>GSAAKMAKNVDKPLFTATFNVQASSADYATFIAGIRNKLRNPAHFSHNRPVLPPVEPNVPPSRWFHVVLKASPTSAGLTLAIRADNIYLEGFKSSDGTWWELTPGLIPGATYVGFGG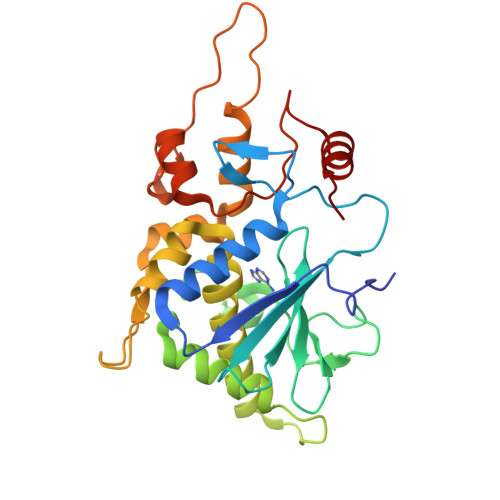TYRDLLGDTDKLTNVALGRQQLADAVTALHGRTKADKPSGPKQQQAREAVTTLLLMVNEATRFQTVSGFVAGLLHPKAVAAASGKIGNEMKAQVNGWQDLSAALLKTDVKPPPGKSPAKFAPIEKMGVRTAVQAANTLGILLFVEVPGGLTVAKALELFHASGGK[4x]N-[4-({[(6S)-2-amino-5-methyl-4-oxo-1,4,5,6,7,8-hexahydropteridin-6-yl]methyl}amino)benzoyl]-L-gamma-glutamyl-L-glutamic 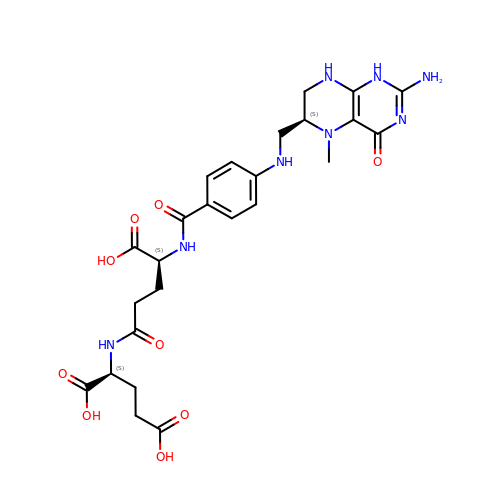acid | C25 H32 N8 O9 | VNEFZDDORGCJSD-JYJNAYRXSA-N> GGLEKDFLPLSFGWFLTKKSSETLRKAGQVFLEELGNHKAFKKELRHFISGDEPKEKLELVSYFGKRPPGVLHCTTKFCDYGKAAGAEEYAQQEVVKRSYGKAFKLSISALFVTPKTAGAQVVLTDQELQLWPSDLDKPSASEGLPPGS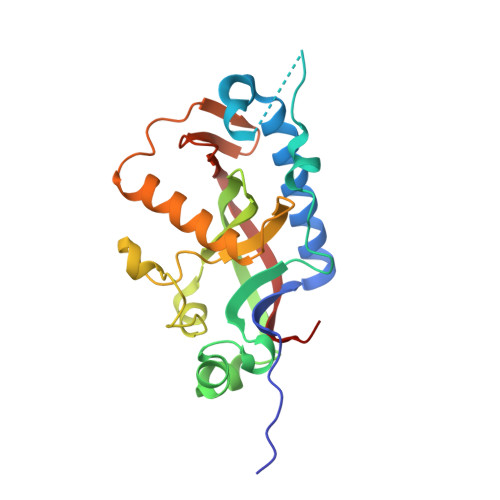RAHVTLGCAADVQPVQTGLDLLDILQQVKGGSQGEAVGELPRGKLYSLGKGRWMLSLTKKMEVKAIFTGYYG> LAVTPDA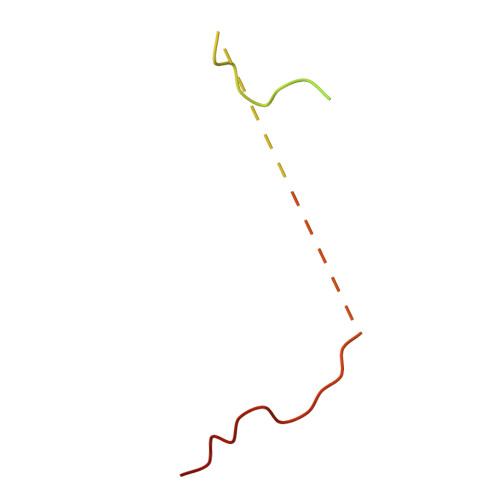ASQPLIDLPLIDFCDTPEAHVAVGSESRPLIDLMTNTPDMNKNVAKPSPVVGQLIDLSSP> GGVSFSEVMGKQKDEQAREQLKEGMIKIEEQGKKLSETRTQEELQKYVAAVATFALQAGFLGPNLE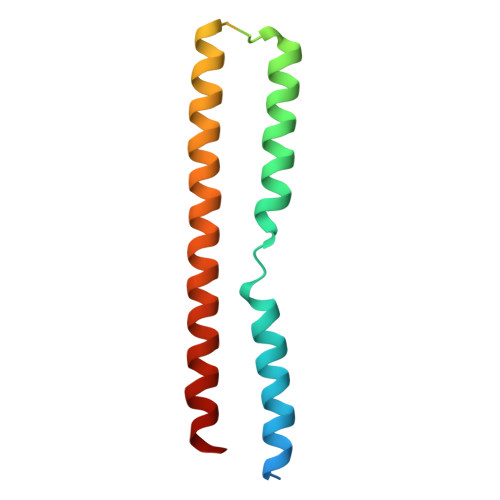ERRGFNRRGKEEIGKISGEVYLKLLDLKKAVRAKEKKGLDILNMVGEIKGTLERVYA>GSKGVSDLLGFKIFGMPLPLYAFALITLLLSHFYNALPTDIVGGFAIMFIIGAIFGEIGKRLPIFNKYIGGAPVMIFLVAAYFVYAGIFTQKEIDAISNVMDKSNFLNLFIAVLITGAILSVNRRLLLKSLLGYIPTILMGIVG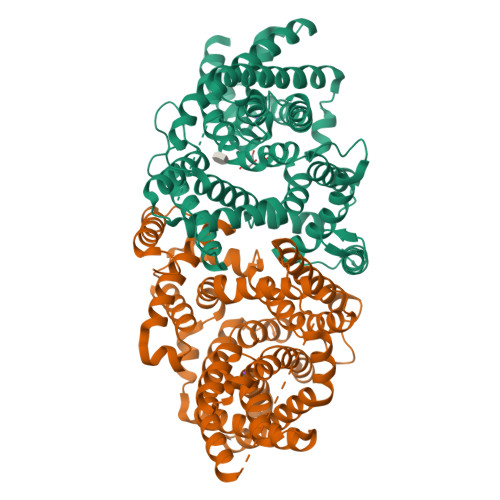ASIFGIAIGLVFGIPVDRIMMLYVLPIMGGGNGAGAVPLSEIYHSVTGRSREEYYSTAIAILTIANIFAIVFAAVLDIIGKKHTWLSGEGELVRKASFKVEEDEKTGQITHRETAVGLVLSTTCFLLAYVVAKKILPSIGGVAIHYFAWMVLIVAALNASGLCSPEIKAGAKRLSDFFSKQLLWVLMVGVGVCYTDLQEIINAITFANVVIAAIIVIGAVLGAAIGGWLMGFFPIESAITAGLCMANRGGSGDLEVLSACNRMNLISYAQISSRLGGGIVLVIASIVFGMMIPR[4x]>XEVEALEKKVEALELKVQKL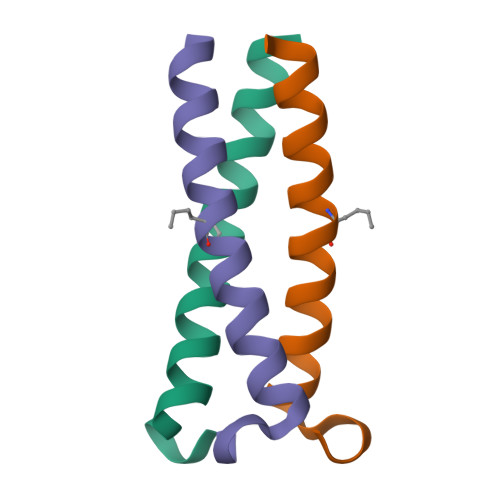EKKVEALEHGWDGR[2x]>MASWSHPQFEKGGSKSALDPVEFLKGALEIPSPSGKERLVAEYLAEGMQKLGLKGFVDEADNARGQVGEGPVQVVLLGHIDTVPGQIPVRLEGGRLFGRGAVDAKGPFVAMIFAAAGLSEEARKRLTVHLVGATEEEAPSSKGARFVAPRLKPHYAVIGEPSGWEGITLGYKGRLLVKARREKDHFHSAHHEPNAAEELISYFVAIKAWAEAMNVGQRPFDQVQYTLRDFRVHPAELRQVAEMFFDLRLPPRLPPEEAIRH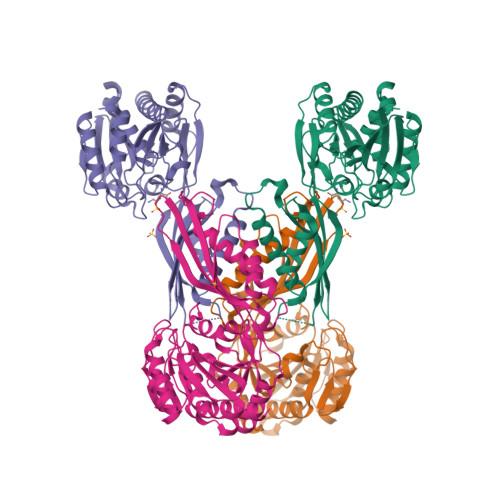LTAYAPPTIELEFFGREVPYQGPKDTPLTRAFRQAIRKAGGRPVFKLKTGTSDMNVLAPHWPVPMVAYGPGDSTLDHTPYEHVEVAEFLKGIEVLRGALEALAQTHAGEKEG[2x]> MRVFHFSKLPLGVAILAASSSVFAVTLDGGAVAAPDQYGAKVAAEILKKGGNAVDAAVATAFTLAVTYPEAGNIGGGGFMTLYVDGKPYFLDYREIAPKAA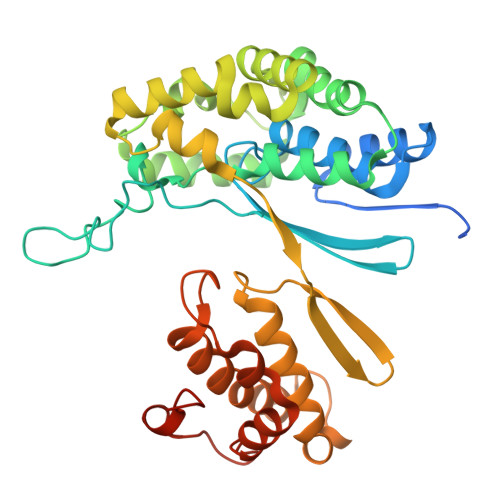TKTMYLNEKGEVIENLSLVGAKAAGVPGTVMGLWEAHQRFGKLKWSELLTPAIGYAQTGFKVADQQYQYRQDAIALFNGKTNFGDYFGTMKPGEVFKQPELAKTLERIADKGPDDFYKGETAKLLIAQMKQDGGLITSDDLVDYQAKWREPMRIDWQGNTLYTAPLPSSGGIALAQLIGIKEQRAADFKGVELNSAKYIHLLSEIEKRVFADRADYLGDPQFSKVPVAQLTDPKYIAKRAGEVNPDAISATEKVRPGLEPHQTTHFSIVD>[3x]MSY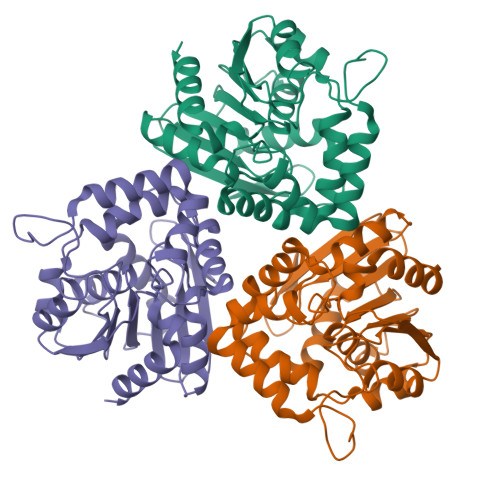VTTKDGVQIFYKDWGPRDAPVIHFHHGWPLSADDWDAQLLFFLAHGYRVVAHDRRGHGRSSQVWDGHDMDHYADDVAAVVAHLGIQGAVHVGHSTGGGEVVRYMARHPEDKVAKAVLIAAVPPLMVQTPGNPGGLPKSVFDGFQAQVASNRAQFYRDVPAGPFYGYNRPGVEASEGIIGNWWRQGMIGSAKAHYDGIVAFSQTDFTEDLKGIQQPVLVMHGDDDQIVPYENSGVLSAKLLPNGALKTYKGYPHGMPTTHADVINADLLAFIRS>GPEFEHDLERLCFIGGYDNDNDKVIVVVTKNLELFKKYDDINLIKEAYNHVHKLIQKDERYTAVFFAHDSTVFSYLGLSLKAYYGMDYYLHKNV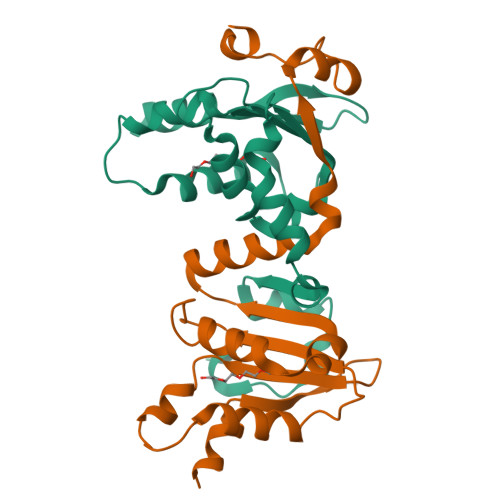KAVYVIHTDWMSKVAIRTLLSIASPKFTRKFRYLNSISDLNKYIPLSHLKLPPIVYEFDRNVEPA[4x]>NGPSPNLPPGFDFTDPAIYAERLPVAEFAELRSAAPIWWNGQDPGKGGGFHDGGFWAITKLNDVKEISRHSDVFSSYENGVIPRFKNDIAREDIEVQRFVMLNMDAPHHTRLRKIISRGFTPRAVGRLHDELQERAQKIAAEAAAAGSGDFVEQVSCELPLQAIAGLLGVPQEDRGKLFHWSNEMTGNEDPEYAHIDPKASSAELIGYAMKMAEEKAKNPADDIVTQLIQADIDGEKLSDDEFGFFVVMLAVAGNETTRNSITQGMMAFAEHPDQWELYKKVRPETAADEIVRWATPVTAFQRTALRDYELSGVQIKKGQRVVMFYRSANFDEEVFQDPFTFNILRNPNPHVGFGGTGAHYCIGANLARMTINLIFNAVADHMPDLKPISAPERLRSGWLNGIKHWQVDYTGRCPVAH[3x]

Breakdown is then initiated with the conversion of the C‐3 hydroxyl group to a ketone (cholest‐4‐en‐3‐one, cholestenone) by the oxidase ChoD, and further oxidation at the C‐26 “tail” region via a three‐step process involving oxidation to the hydroxyl, aldehyde, and carboxylic acid species. These sidechain‐modifying reactions are catalysed by the cytochromes P450 CYP125A1 and CYP142A1 (CYP125 and CYP142 hereafter). Comparison of the effect of complementing a CYP125 knockout in the CDC1551 strain of Mtb (which does not express the CYP142 protein), with CYP125 or CYP142 reveals that the two enzymes are functionally redundant with respect to growth on cholesterol. Here we present a series of compounds based on an ethyl 5‐(pyridin‐4‐yl)‐1H‐indole‐2‐carboxylate pharmacophore which bind strongly to both Mtb cholesterol oxidases CYP125 and CYP142.

To overcome these issues, the cyclohexyl group was substituted with piperazine and morpholine rings, compounds 10–12, leading to enhanced solubility. Upon inspection of the corresponding CYP125 ligand complex X‐ray crystals structures, it was noted that elaboration from the R1 position (N of the indole) dramatically changes the binding pose of this series. In the cases of compounds 7, 8, 10, and 12 the ligand is observed at a greater distance from the heme, typically with the pyridine coordination mediated via a water molecule, to produce a reverse‐type I interaction similar to what was observed for the inhibitor LP10. R1 position are observed significantly closer to the heme iron, with compound 10 observed at 2.4 Å from the distal water. This is likely attributable to the ability of the additional carbon to facilitate positioning of the ring closer to the plane of the indole, as opposed to compounds 7 and 8 which extend at an angle of 67° from this plane because of the geometric requirements of the single carbon linker. Later compounds such as 10, 12, and 19 have been optimized towards the observed pose of 7 and 8 in CYP125, with changes that gave improved solubility also allowing more favourable interactions with the more polar environment around Asn203, Glu204, the carboxyl oxygen of Arg99, and the N−H of Trp414.> MTVAYIAIGSNLASPLEQVNAALKALGDIPESHILTVSSFYRTPPLGPQDQPDYLN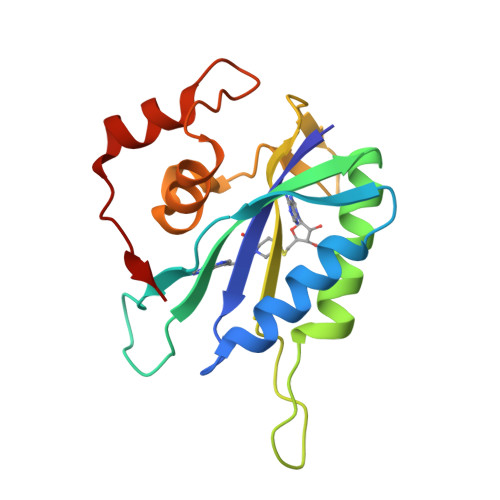AAVALETSLAPEELLNHTQRIELQQGRVRKAERWGPRTLDLDIMLFGNEVINTERLTVPHYDMKNRGFMLWPLFEIAPELVFPDGEMLRQILHTRAFDKLNKW>[2x]GSLSRLSYKSNNNSFVLGIGISVPGEPISQQSLKDSISNDFSDKAETNEKVKRIFEQSQIKTRHLVRDYTKPENSIKFRHLETITDVNNQFKKVVPDLAQQACLRALKDWGGDKGDITHIVSVTSTGIIIPDVNFKLIDLLGLNKDVERVSLNLMGCLAGLSSLRTAASLAKASPRNRILVVCTEVCSLHFSNTDGGDQMVASSIFADGSA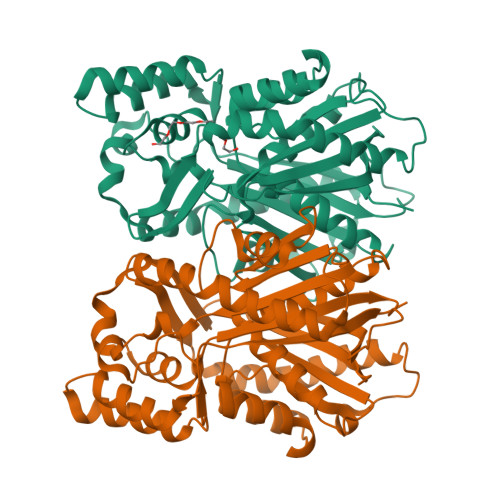AYIIGCNPRIEETPLYEVMCSINRSFPNTENAMVWDLEKEGWNLGLDASIPIVIGSGIEAFVDTLLDKAKLQTSTAISAKDCEFLIHTGGKSILMNIENSLGIDPKQTKNTWDVYHAYGNMSSASVIFVMDHARKSKSLPTYSISLAFGPGLAFEGCFLKNVV> R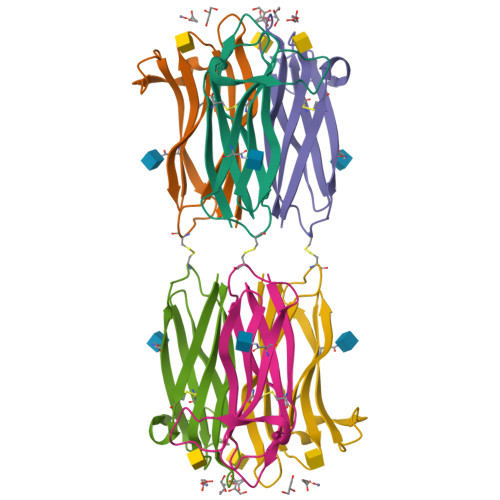VQSGKIDCGDDAGWAKVPSDDPGRDNTRELAKNITFASPYCRPPVVLLSITQLDVEQSQNLRVIARLYSVSPSGFKASCYTWHNTKVYSMSISWISIENY> MAGHSHWAQIKHKKAKVDAQRGKLFSKLIREIIVATRLGGPNPEFNPRLRTAIEQAKKANMPWENIERAIKKGAGELEGEQFEEVIYEGYAPGGVAVMVLATTDNRNRTTSEVRHVFTKHGGNLGASGCVSYLFERKG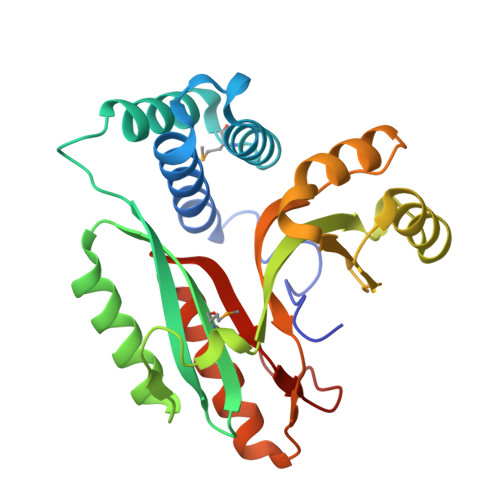YIEVPAKEVSEEELLEKAIEVGAEDVQPGEEVHIIYTVPEELYEVKENLEKLGVPIEKAQITWKPISTVQINDEETAQKVIKLLNALEELDDVQQVIANFEIPEEILQKVG> MHRVMGIETEYGISVPHQPNANAMAASSQVVNAYAPIGAPAQRQARWDFEEENPLRDARGFEVAREAADPSQLTDEDLGLANVILTNGARLYVDHAHPEYSTPEVTNPRDAVLWDKAGERIMAEAARRAADLPMGWTIQLYKNNTDNKGASYGCHENYLMNRSTPFADIVRHLIPFFVTRQVFCGAGRVGIGADGRGEGFQLSQRADFFEVEVGLETTLKRPIINTRDEPHADPEKYRRLH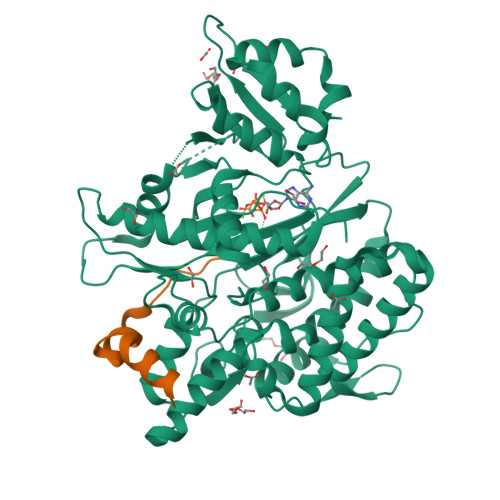VIIGDANMSEIATYLKLGTTALVLAMIEDGFLSQDFSVESPVGALRAVSHDPTLRYQLRLHDGRRLTAVQLQMEYLEQARKYVEDRFGTDVDDMTRDVLDRWETTLVRLADDPMQLSRDLDWVAKLSILEGYRQRENLPWSAHKLQLVDLQYHDVRPDRGLYNRLVARGRMNLLVDEAAVRTAMHEPPNDTRAYFRGRCLAKFGAEIAAASWDSVIFDLPGRDSLQRVPTLEPLRGTRAHVGDLLDRCRSATELVAALTGGENLYFQ;> DAILDEIDDVLEENAEEFVRSYIQKGGQ>HGFVQNIVIDGKNYGGYLVNQYPYMSNPPEVIAWSTTATDLGFVDGTGYQTPDIICHRGAKPGALTAPVSPGGTVELQWTPWPDSHHGPVINYLAPCNGDCSTVDKTQLEFFKIAESGLINDDNPPGIWASDNLIAA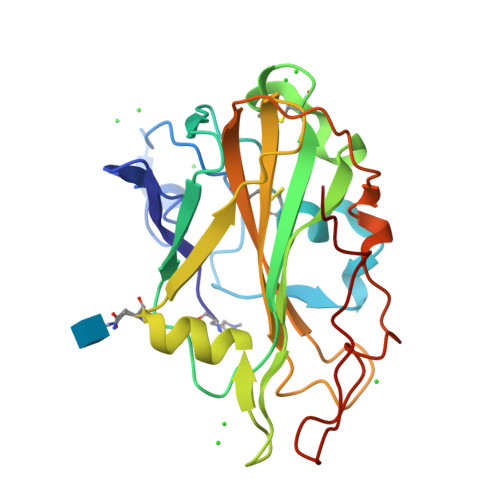NNSWTVTIPTTIAPGNYVLRHEIIALHSAQNQDGAQNYPQCINLQVTGGGSDNPAGTLGTALYHDTDPGILINIYQKLSSYIIPGPPLYTG[2x]>MSYYHHHHHHLESTSLYKKAGLQALLLEQQDGKTLASVQTLDESRLPEGDVTVDVHWSSLNYKDALAITGKGKIIRNFPMIPGIDFAGTVRTSEDPRFHAGQEVLLTGWGVGENH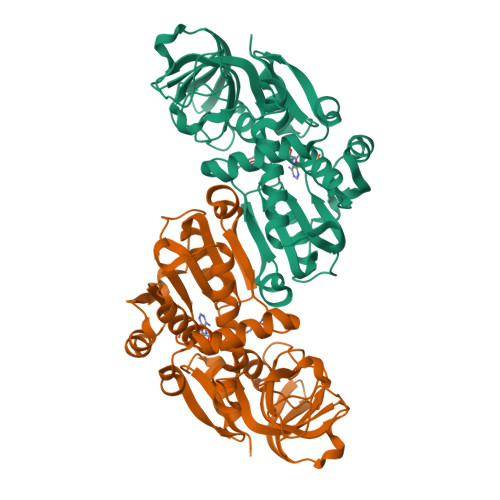WGGLAEQARVKGDWLVAMPQGLDARKAMIIGTAGFTAMLCVMALEDAGVRPQDGEIVVTGASGGVGSTAVALLHKLGYQVVAVSGRESTHEYLKSLGASRVLPRDEFAESRPLEKQVWAGAIDTVGDKVLAKVLAQMNYGGCVAACGLAGGFTLPTTVMPFILRNVRLQGVDSVMTPPERRAQAWQRLVADLPESFYTQAAKEISLSEAPNFAEAIINNQIQGRTLVKVN[4x]Prinomastat | C18 H21 N3 O5 S2 | 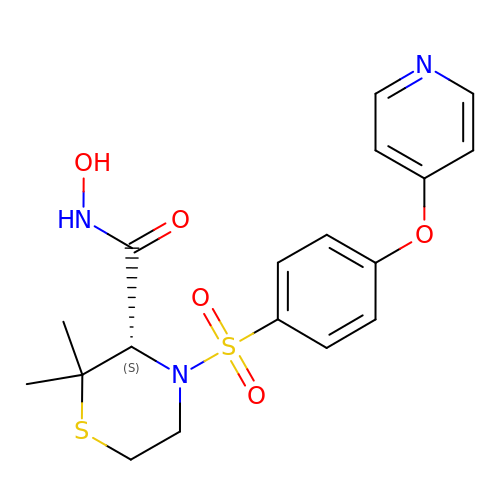YKPYIPVDTNNYCN-INIZCTEOSA-N Leucine-rich repeat-containing G protein-coupled receptor 4 (LGR4) plays a critical role in regulating the wingless-related integration site (Wnt) signaling pathway and is essential for organ development and carcinogenesis. LGR4, along with its ligand R-spondin (RSPO), potentiates Wnt/β-catenin signaling by recruiting its signaling suppressor, E3 ligase Zinc and Ring Finger 3 (ZNRF3), and inducing its membrane clearance. Cell surface-expressed LGR4/5, members of the class A G-protein coupled receptors (GPCR) family, have an extracellular domain (ECD) comprising 17 leucine-rich repeats (LRRs), followed by a seven-transmembrane domain (TMD), and an intracellular domain (ICD). ZNRF3/RNF43, LGR4, and RSPO form a ternary complex on the cell surface, which relieves ZNRF3/RNF43-mediated suppression of Wnt/β-catenin signaling and thereby potentiates pathway activation.

We purified LMNG/CHS detergent-solubilized ternary complexes of human LGR4, RSPO2, and ZNRF3 (residues 56-267, ECD-TMD) from Expi293F cells cotransfected with LGR4, RSPO2, and ZNRF3. Cryo-EM analysis of this sample revealed two distinct LGR4–RSPO2–ZNRF3 complexes with stoichiometric ratios of 1:1:2 and 2:2:2, corresponding to a heterotetramer and a heterohexamer, respectively. We obtained cryo-EM maps of LGR4-RSPO2-ZNRF31:1:2 heterotetramer and LGR4-RSPO2-ZNRF32:2:2 heterohexamer to resolutions of 3.2 Å and 3.5 Å, respectively. In the LGR4-RSPO2-ZNRF31:1:2 complex, RSPO2 was bound to one protomer of the ZNRF3 dimer through which LGR4 was associated, forming a 1:1:1 complex on one side of the structure. No apparent interactions occurred between the ECDs of ZNRF3 and LGR4 in the 1:1:1 assembly. However, ZNRF3 made contact with LGR4*, thereby stabilizing the overall complex, particularly ZNRF3 dimerization. At the center of the interface, ZNRF3 Y77 and T78 formed hydrogen bonds with G435 and N437 of LGR4*, respectively. In addition, two pairs of electrostatically complementary residues (E67 of ZNRF3 and R392 of LGR4* and E62 of ZNRF3 and R460 of LGR4*) located at the peripheral regions of the interface might support this interaction. In the LGR4-RSPO2-ZNRF31:1:2 structure, the TM helix of only one protomer, ZNRF3*, was defined by the cryo-EM density, whereas that of the other protomer, ZNRF3, was not visible, indicating that the TM helices of ZNRF3 are flexible. The observed TM helix of ZNRF3* was aligned and in contact with TM1 and TM7 of LGR4 on the extracellular side of the membrane but made no contact on the intracellular side.

> MPGPLGLLCFLALGLLGSAGPSGAAPPLCAAPCSCDGDRRVDCSGKGLTAVPEGLSAFTQALDISMNNITQLPEDAFKNFPFLEELQLAGNDLSFIHPKALSGLKELKVLTLQNNQLKTVPSEAIRGLSALQSLRLDANHITSVPEDSFEGLVQLRHLWLDDNSLTEVPVHPLSNLPTLQALTLALNKISSIPDFAFTNLSSLVVLHLHNNKIRSLSQHCFDGLDNLETLDLNYNNLGEFPQAIKALPSLKELGFHSNSISVIPDGAFDGNPLLRTIHLYDNPLSFVGNSAFHNLSDLHSLVIRGASMVQQFPNLTGTVHLESLTLTGTKISSIPNNLCQEQKMLRTLDLSYNNIRDLPSFNGCHALEEISLQRNQIYQIKEGTFQGLISLRILDLSRNLIHEIHSRAFATLGPITNLDVSFNELTSFPTEGLNGLNQLKLVGNFKLKEALAAKDFVNLRSLSVPYAYQCCAFWGCDSYANLNTEDNSLQDHSVAQEKGTADAANVTSTLENEEHSQIIIHCTPSTGAFKPCEYLLGSWMIRLTVWFIFLVALFFNLLVILTTFASCTSLPSSKLFIGLISVSNLFMGIYTGILTFLDAVSWGRFAEFGIWWETGSGCKVAGFLAVFSSESAIFLLMLATVERSLSAKDIMKNGKSNHLKQFRVAALLAFLGATVAGCFPLFHRGEYSASPLCLPFPTGETPSLGFTVTLVLLNSLAFLLMAVIYTKLYCNLEKEDLSENSQSSMIKHVAWLIFTNCIFFCPVAFFSFAPLITAISISPEIMKSVTLIFFPLPACLNPVLYVFFNPKFKEDWKLLKRRVTKKENLYFQGDYKDDDDKHHHHHHHH;>[2x]METGLRWLLLVAVLKGVQCKETAFVEVVLFESSPSGDYTTYTTGLTGRFSRAGATLSAEGEIVQMHPLGLCNNNDEEDLYEYGWVGVVKLEQPELDPKPCLTVLGKAKRAVQRGATAVIFDVSENPEAIDQLNQGSEDPLKRPVVYVKGADAIKLMNIVNKQKVARARIQHRPPRQPTEYFDMGIFLAFFVVVSLVCLILLVKIKLKQRRSQNSMNRLAVQALEKMETRKF;> MQFRLFSFALIILNCMDYSHCQGNRWRRSKRASYVSNPICKGCLSCSKDNGCSRCQQKLFFFLRREGMRQYGECLHSCPSGYYGHRAPDMNRCARCRIENCDSCFSKDFCTKCKVGFYLHRGRCFDECPDGFAPLEETMECVEENLYFQGHHHHHHHHHH> MAVQILRDRSRAAVQKVVLGATKDQGGTRSHTIVVGGDAALPFHHFEGEIVNRPVIGMEVQDIVPDW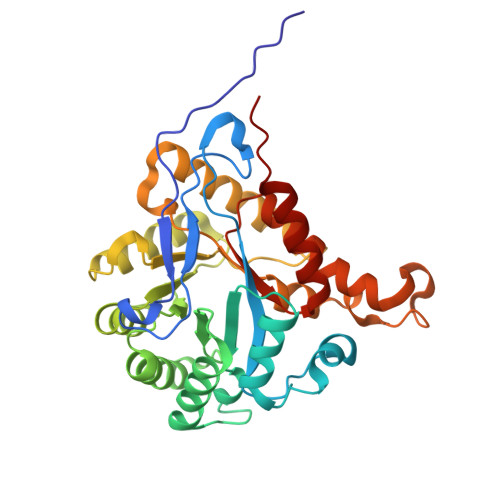PDVLKDPFTDVINEPGRWAQKCVAEYGADLIYLKLDGADPEGANHSVDQCVATVKEVLQAVGVPLVVVGCGDVEKDHEVLEAVAEAAAGENLLLGNAEQENYKSLTAACMVHKHNIIARSPLDINICKQLNILINEMNLPLDHIVIDPSIGGLGYGIEYSFSIMERIRLGALQGDKMLSMPVICTVGYEAWRAKEASAPVSEYPGWGKETERGILWEAVTATALLQAGAHILLMRHPEAVARVKENIDQLMVSNAY> ERAGPVTWVMMIACVVVFIAMQILGDQEVMLWLAWPFDPTLKFEFWRYFTHALMHFSLMHIL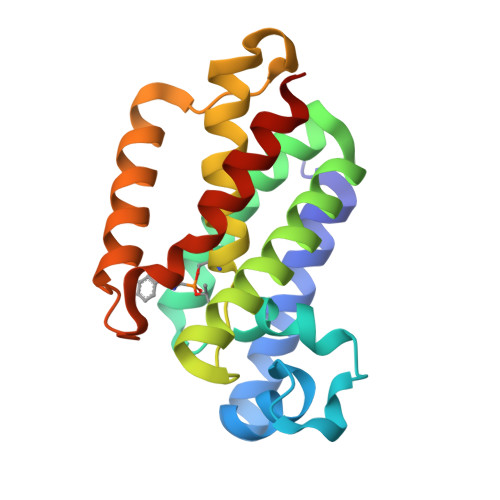FNLLWWWYLGGAVEKRLGSGKLIVITLISALLSGYVQQKFSGPWFGGLSGVVYALMGYVWLRGERDPQSGIYLQRGLIIFALIWIVAGWFDLFGMSMANGAHIAGLAVGLAMAFVDSLNA>[3x]DSKTVNYFDIITIKHQDTDAFLHSHLARYPQRYEDGRISSAGQQVTGYTHPDFNNQWEVLPPHGSDVGKGQAVL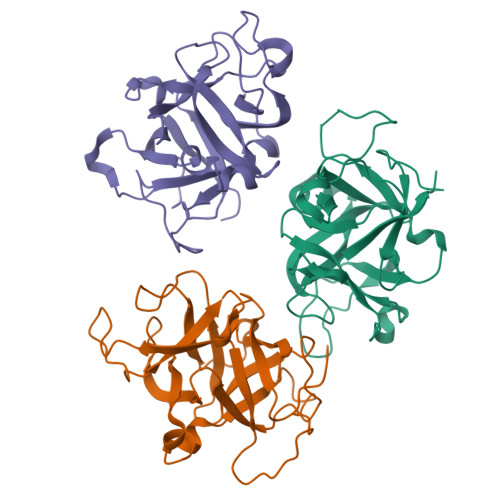LNQHIRLRHVATDTYLLAHDVASPFYPTNEEITTVTLEEGDGELYPETLFAFQPLKKSDEGHVLKSKTVSFRLFHVDTSVALWTHNDELLPDWGFQQQEINGNKKVIDPSNNWVVDEIVNL>[2x]GAMSLGKRLKE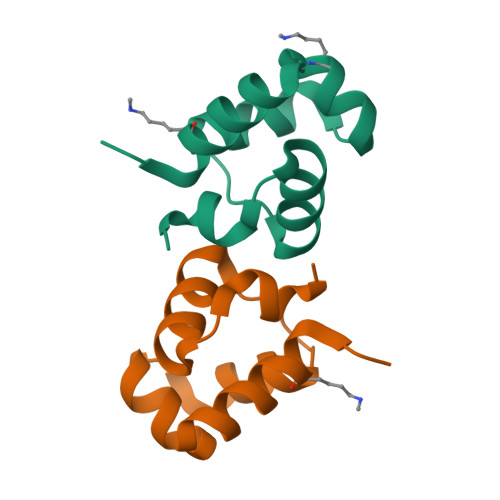ARQKAGYTQKEAAEKLNIGNNNLSNYERDYRDPDTDTLLKLSNLYNVSTDYLLGK> MTENILRKSDEEIQKEITARVKALESMLIEQGILTTSMIDRMAEIYENEVGPHLGAKVVVKAWTDPEFKKRLLADGTEACKELGIGGLQGEDMMWVENTDEVHHVVVCTLCTCYPWPVLGLPPNWFKEPQYRSRVVREPRQLLKEEFGFEVPPSKEIKVWDSSSEMRFVVLPQRPAGTDGWSEEELATLVTRESMIGVEPAKAV;> MNGVYDVGGTDGLGPINRPADEPVFRAEWEKVAFAMFPATFRAGFMGLDEFRFGIEQMNPAEYLESPYYWHWIRTYIHHG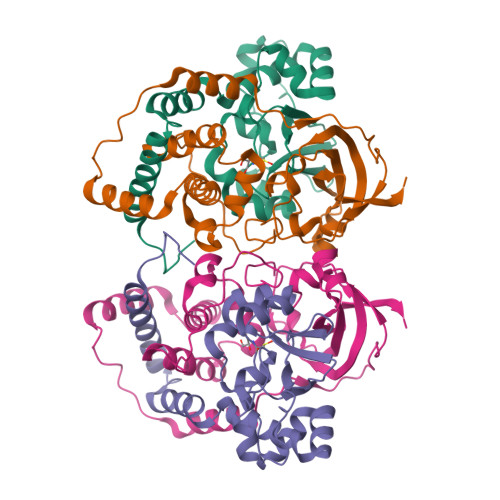VRTGKIDLEELERRTQYYRENPDAPLPEHEQKPELIEFVNQAVYGGLPASREVDRPPKFKEGDVVRFSTASPKGHARRARYVRGKTGTVVKHHGAYIYPDTAGNGLGECPEHLYTVRFTAQELWGPEGDPNSSVYYDCWEPYIELVDT> IHRTQHW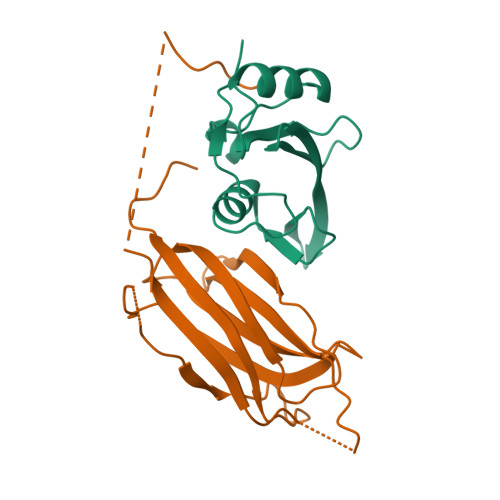FHGRISREESHRIIKQQGLVDGLFLLRDSQSNPKAFVLTLCHHQKIKNFQILPCEDDGQTFFSLDDGNTKFSDLIQLVDFYQLNKGVLPCKLKHHCIRVAL;> ELHNDDTRVVRVKVIAGIGLAKKDILGASDPYVRVTLYDPMSGILTSVQTKTIKKSLNPKWNEEILFRVLPQRHRILFEVFDENRLTRDDFLGQVDVPLYPLPTENPRMERPYTFKDFVLHPRSHKSRVKGYLRLKMTYLPKNGSEDENADQAEELEPGWVVLDQPDAATHLPHPP>[8x]MHHHHHHMSTKDLIETCCAAGQQWAIDNDECQEIPENGAQSDICRIAQRQCCISYLKEKSCVAGVMGAKEGETCGAEDNDTCGVSLYKQCCDCCGLGLRVRAEGQSCESNPNLGYPCNHVMLSCCEG

Fibulin-2 is a multidomain, disulfide-rich, homodimeric protein which belongs to a broader extracellular matrix family. It plays an important role in the development of elastic fiber structures. Malfunction of fibulin due to mutation or poor expression can result in a variety of diseases including synpolydactyly, limb abnormalities, eye disorders leading to blindness, cardiovascular diseases and cancer. The three anaphylatoxin-like modules (C435-C543) following the N-domain are also found in fibulin-1, but not in other fibulins.

We were able to obtain diffracting crystals and solved the structure in the P21 space group at 2.2 Å resolution. The structure included four dimers (AB, CD, EF and GH) in the asymmetric unit, with each dimer in a local two-fold symmetry. The overall structure of each chain is predominantly α-helical, which is consistent with the CD data. There are four alpha helices (T428-D445 for α1, D460-E488 for α2, L504-A520 for α3, Y533-E544 for α4) which all run in the same direction. The loop structures between α1 and α2 (N446-S459) and between α2 and α3 (G499-S503) were incompletely modelled in all 8 chains indicating the flexible nature of these regions. The structure has a disulfide bond architecture which stabilizes the three anaphylatoxin modules. In total, 8 intra-molecular disulfide bonds are found in the domain. All of this suggests that in fibulin-2, the three anaphylatoxin modules are all embedded into a single-domain four-helix structure forming a dimer with covalent bonding via C500. Cys500 locates in the flexible α2-α3 loop, which is only partly visible in the electron density maps. When combined with the non-reducing SDS-PAGE and MS, which both indicate that all of the protein is in a disulfide linked homodimer, the crystal structure data implies that the inter-subunit disulfide is formed, but that it is not stabilizing the flexible nature of the α2-α3 loop.> MSMLKREDWYDLTRTTNWTPKYVTENELFPEEMSGARGISMEAWEKYDEPYKITYPEYVSIQREKDSGAYSIKAALERDGFVDRADPGWVSTMQLHFGAIALEEYAASTAEARMARFAKAPGNRNMATFGMMDENRHGQIQLYFPYANVKRSRKWDWAHK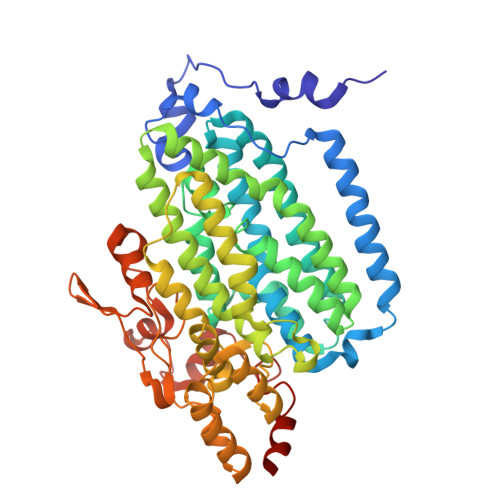AIHTNEWAAIAARSFFDDMMMTRDSVAVSIMLTFAFETGFVNMQFLGLAADAAEAGDHTFASLISSIQTDESRHAQQGGPSLKILVENGKKDEAQQMVDVAIWRSWKLFSVLTGPIMDYYTPLESRNQSFKEFMLEWIVAQFERQLLDLGLDKPWYWDQFMQDLDETHHGMHLGVWYWRPTVWWDPAAGVSPEEREWLEEKYPGWNDTWGQCWDVITDNLVNGKPELTVPETLPTICNMCNLPIAHTPGNKWNVKDYQLEYEGRLYHFGSEADRWCFQIDPERYENHTNLVDRFLKGEIQPADLAGALMYMSLEPGVMGDDAHDYEWVKAYQKKTNAA>[2x]MEGGPALFQSDMTFKIF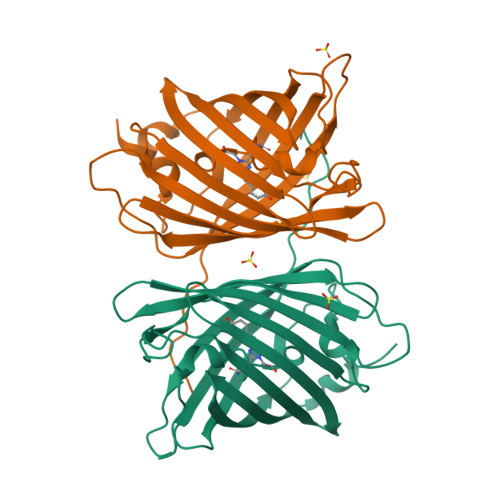IDGEVNGQKFTIVADGSSKFPHGDFNVHAVCETGKLPMSWKPICHLIQYGEPFFARYPDGISHFAQECFPEGLSIDRTVRFENDGTMTSHHTYELDDTCVVSRITVNCDGFQPDGPIMRDQLVDILPNETHMFPHGPNAVRQLAFIGFTTADGGLMMGHFDSKMTFNGSRAIEIPGPHFVTIITKQMRDTSDKRDHVCQREVAYAHSVPRITSAIGSDED>GYTLWNDQIVKDEEVKIDKEDRGYQFGDGVYEVVKVYNGEMFTVNEHIDRLYASAEKIRITIPYTKDKFHQLLHELVEKNELNTGHIYFQVTRGTSPRAHQFPENTVKPVIIGYTKENPRPLENLEKGVKA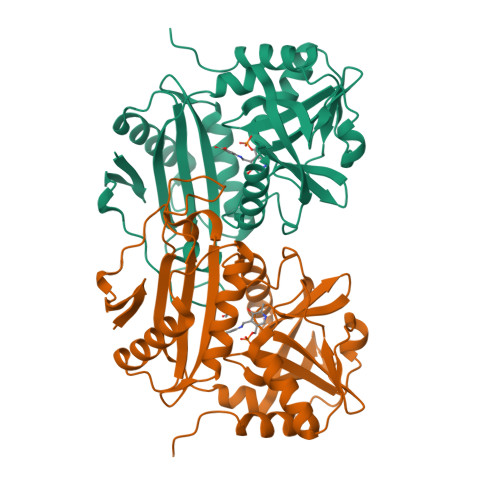TFVEDIRWLRCDIKSLNLLGAVLAKQEAHEKGCYEAILHRNNTVTEGSSSNVFGIKDGILYTHPANNMILKGITRDVVIACANEINMPVKEIPFTTHEALKMDELFVTSTTSEITPVIEIDGKLIRDGKVGEWTRKLQKQFETKIPKPL[2x]> GAMGSGIPMEASPHIRYAFQNDKLLLQQASVGRLTLVNKTTILLRPMKTTTVDLGLYARPPEGHGLMLWGSTSRPVTSHVGIIDPGYTGELRLILQNQRRY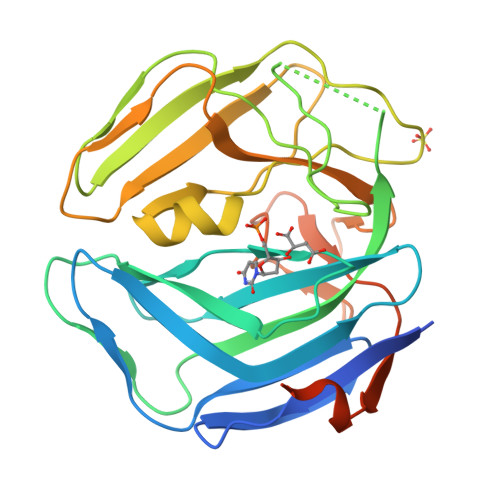NSTLRPSELKIHLAAFRYATPQMEEDKGPINHPQYPGDVGLDVSLPKDLALFPHQTVSVTLTVPPPSIPHHRPTIFGRSGLAMQGILVKPCRWRRGGVDVSLTNFSDQTVFLNKYRRFCQLVYLHKHHLTSFYSPHSDAGVLGPRSLFRWASCTFEEVPSLAMGDSGLSEALEGRQGRGFGSSGQ> MDAATILSDLSTIKTDINTLTQHFNEFTGDLLQALAAQAVEQQLESDIDQATADAKATSALSAADSTSVTNALLGLKPDIVTSLDAIV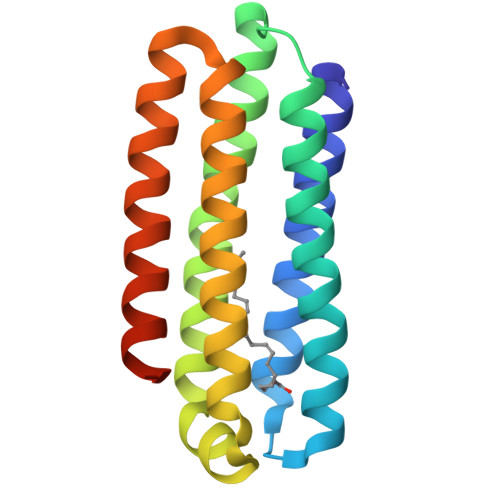AKKPQVDSAGVGSLVLSDLNALQSKTDALSGALQDIATATDKDTIASGTQDIDAAFSSAIAVFSLEHHHHHH Here we present the cryo-EM structure of an early ancestor in the evolution of complex I, the elemental sulfur (S0)-reducing reductase MBS. MBH and MBS are found in the anaerobic hyperthermophilic archaeon Pyrococcus furiosus, which oxidizes the redox protein ferredoxin, produces H2S or H2, and conserves energy by pumping Na+. MBS reductively cleaves linear polysulfide chains (Sn2−, where n ≥ 4), produced abiotically from the reaction of H2S and S0 (Eq. 1) in the hydrothermal vent environments that P. furiosus inhabits, into two shorter polysulfides (Eq. 2). MBS contains two proton pumps compared to one in MBH and likely conserves twice the energy.

We determined the cryo-EM structure of MBS in a dimer complex form. The atomic model contained 26 protein subunits and 116 transmembrane helices (TMHs). The MBS monomer consists of a peripheral cytoplasmic arm (MbsJ, K, L, and N), anchored to the membrane by MbsM, and coordinates three [4Fe-4S] clusters that transfer electrons from ferredoxin to the substrate polysulfide. The MBS dimer complex is assembled via extensive contacts at two main places between the proximal membrane module of one MBS and the membrane-anchored peripheral module of the other. The second contact involves the tryptophan-rich C-terminal extension (W90, W91, and W94) of MbsD of one MBS projecting into a largely hydrophobic cleft in the peripheral domain of the other. In MBS, a large hydrophobic chamber, similar in size to those in MBH and complex I, is formed by cytoplasmic MbsL, MbsJ, and their membrane anchor MbsM. The proximal (p-)[4Fe-4S] cluster in MBS and complex I is at the top of the hydrophobic chamber but, in stark contrast to that in complex I (and MBH), the MBS p-[4Fe-4S] is coordinated by only three rather than the expected four cysteines (C28, C93 and C123 of MbsJ). In MBS, this structural motif is three residues shorter than it is in MBH, leaving one of the cysteines (MbsJ C25) no longer able to participate in cluster coordination. The unique Fe atom of its p-[4Fe-4S]2+ cluster binds polysulfide (Sn2−), accepts an electron from the medial (m-)[4Fe-4S]1+ cluster and catalyzes the two-electron reduction of an internal disulfide, generating two smaller polysulfides (Sn-x2- and Sx2-) and the superoxidized form of p-[4Fe-4S]3+.

>MEEASSISRYLYTFIVLFIIWLFLTASLDPQELTIGALFSAIAALFTYEIFTTRGLANLHPKRVLYFIAYIPYFLWAMIMANLDVAYRVLHPKRPINPGIVECKTTLTNNVGKMALANSITLTPGTITLDVDGDKYFIHWIDVKDSSVEGASEHITKPFEKFLRVIFE[2x];>[2x]MIGVNIYLLLIGVATLLSMYRVFRGPTTVDRLVAVDIMTTITVGLMVLFALYYRRIIFLDVALVYAILSFAGVIAFARYLEGGL;>[2x]MSVLSLIGELLVLFGTVFYLLSTLGLIRMPDVYNRMQTATKSATLGSLGVIIGTGIWALGEGFSVAWLTKAIVIAAFLLLTNPISAHALIRAAYKSGIPLWEGSVVDKYKEHLERKKKEEGEQE;>MNCIVCIEYIIVALMIISAILAVEWRDLLASTVGMAAVSLFASILFFFLQAPDVAMTEAAIGAALSAAVFIFAIKRTYRYETEEEEKLGWWVRW[2x];>[2x]MLKRVLAILTILVIGYWLAQGLADVPFGQDKMVVGKYYLEHVKEETGAVNAVTAVVVNYRGLDTLGEVTVLFIASTGVAALLWKKKRERTAKTEGSVVLTTGARLLFPFIALFGMYIFIHGHLTPGGGFPGGATIATAFLLMYLAFTIYEIPHRGFEVTEGLAGMGYVITGLIGLAIGGYFLFDWIWQTWGWGHENIGRLFSGGFIPIIYTLIGIKVGTELSGIVDNMLKEEVKE;>MISSYYFGAISLILIGLYAVLVKKNLLKILIGLSIMETGVNLLLISIGYVSGKSAPILSEGVTASNAVDPIPQALVLTAIVIGVATTAMALSVAILLYEKYGTLNIEEIRRLRG[2x];>MSQVAALLIALPLISAFFVPVLKQIGKSLIKPFLVIITLLQTLIASWAFVQVYSTGKPIIIYAGGWKPPIGINLYIGHFAALFILVIAVVSFLMALFNFKAVTVEPIDKYAMLFLLLLLGATGMIATGDIFNLFVFMEITAISAYALTAYNKTGEAAEASMKYIVLGGIGSSFFLVGVALIYGATGTLNMAHLAMLANDINPTVVQVGLALIIFGLAVEAELFPLNAWAPDAYQAAPHPITVMFSAFVVKAGLYAMARILYLFKDVSGWSSLTKLLIAMATLTVVFAELSALRQKNVKRMIAYSSIGQVGLIALALSLGTQEGVSAGVFHMLNHAIVKTMMFMAIGYVGITLGGTMIENFEGLGKRMPLTSLSLTIGGIATVGVPLFNVFWSKLRIILAAAHEGNLWPVALVLFASVVEAVYYFRLIHTMWFKGKSGERIPEGAIAIVLLLLAMLIIVIGVYPTPFWNLVTKAGSDIVEVSKYVANVLPGVKL[2x];>MVDWRLFEPLFNWARKKSLWIVAFCTGCGGIEMPPLMTARYDLERFGIMPDPSPRQYDLFLITGYVTPKTLKRIIITYEMAPDPKYVLAHGSCPINGGIYWDAYNAIKQLDKYIPVDVYIAGCMPRPEAVMDGIKKLMEMIENGEADGWKRYKENYEWYRKNQDELLGEGWREKEARKWIPWLMDKRKEVKE[2x];>[2x]MTWEKGEEIVKQILEKAPYAEGKVRRERRLEFRVPADKIRDFLRIMKESNFPLMLQITAVDWPKEGEIELVYHLINVELGTHAMVKTRIPRDLDKARMPTVKDIYPAAETYERDVHDFFGVYFEGNEKMEMPWILDDPERGLYPHRKDFDMLAYVKKKYKILDRFDEDKDKYVI;>[2x]MVSQEELIREARQNGMELYPIDKDTYELFFGPQHMATENFSIILKMDGNRVVKAIANPGFLHRGFEKLAEYRPWYTNIALLLRICVPEPDVPEAIYSMAVDEIIGWEVPERAQWIRTLVLEMARVTAYLFWIMGLSFKLGVYTAGQWAAAYRERFMALFEQLTGARVYHIYTIPGGVRRDIPGDKWLRQVRDTVEYLKDKLKDFDNVLFENYITYKRLEGIGVMDKKFALEEGVTGPNLRATGVAYDVRKSDPYLLYPELDFEIPVLKEGDALARVLVRRYELEQDLYIIEQLLDMGPPSGPYKVQDPKLKNLPRFKVPPGEAFAHVEATKGDFGAYVVSDGGHKPYRVHIRGPSIAHGVRVLEQLLVGARLADVPAILMSLDNCPPDIDR;>[2x]MIGVFLRALLIIIYATFVGFIFMGIIRKVTARIHRRIGPPIYQPIIDTLKFFGKKENITHGLIYDFGIIYAVGATILALMFIPLGPISVLRAYGDLILVTFLLEIPMLGIMFAAMSSGNPYAGIGAQRALLTLLAIQVPLGLAIIAVAEYYGTFSTYEIVMAQQKMGWSIFHLPLLLAAIAYDIVLQAMFGKEPFDIMIAPGEISLGPMVEFGGKHMGMLQIQHAMALFAETLFFSNIFLGGGVVTAFGSPLLNTLASLAVLLVKQIAVLLIAIFVGAIFPRFTIDQAAKFYWKWPTIIAAIGAIMASL;>MEEVTFRIAPEEKVKKKPSFLKPWFGLKYLFKKPVTIKIPYEFIEPAPRYRGFHTLDWKKCIGCNMCGQICPARAIEMTWIEGEKRPHPKIDYGRCTFCQFCVDVCPTGALGFIETYMLTTTWREEELLLYDWVPIEPEKFKEIQEKFKDYKFPVEKIEFNKETKEVTYYLRDGTTFKFKILGYGLKPPVKPQPTTKQQEEEKKESGQ[2x];>MNELPIILLSPLIGGALAWLIRVKGIREAIGVVSSAIPLYFLIKLYPALEGEPIRYSLNVGGFELTLALSHISWIFAMIAAVVGLSAVLGLVSTAKDSNEWLFALMSLAGALGVFLANDFVVFFLSWEIMTFASFMMVFKYNRHASLKYFVLSIAGAYAMLLAIGIIYAKTGSLSFPEISAIFRQDAMMGMMGGGGVFTKTETLLIYALFLVAFGVKAGMFPLHVWAPDAYSETNQSYTAMFSGVLSKTGVYGFFLLYLLMYGKLAITLGNVRSAPTFGYIIAFLGGLTIMVGGILAALQEDIRKLFAYSSISQIGYILIGLGIGTPLGIAAATYHAISHALFKGLFFLIVATIIYRTGKTEFKDYGGLAEKMPITFAMAFVAILSLAGIPPMAGFASKWLIFEAVISRNLPILGAMVFFGSAIGFVYLIRFTYAVWFGQRPSDLEDVKDAPLPLAIGMGILAILNVIFGVAPGLVARELNKLFSNPPIGGTIWELDLGFGRYNGLLLSIWLVIGLIIAAILYFMGAGVRKVPVTDTYQSGNPVTMEYNLTIRRNFFLPLKEAMAFWLKMSFDRLYHDIWKAIEELADLARSYVYNGNIQAYAWYLAIILLILVAMGV[2x]>ATFLIWPIYPKIEANEKATAVWLQNTGKTDAMVQIRVFKWNQDGLKDNYSEQSEIIPSPPVAKIKAGEKHMLRLTKSVNLPDGKEQSYRLIVDELPIRLSDGNEQDASKVSFQMRYSIPLFAYGKGIGSGLTEESQKLNAKNALAKPVLQWSVRNNQQGQSELYLKNNGQKFARLSALKTSKTGNDISLGKAAFGYVLSNSTVKFAIDQSTAHELAKTSKIYGVDSSGIKQELIEITKMEDPSGHHHHHH[2x];>[2x]ACSVSASGTSSISVPSIYLMENGENSSQFNSGLSCTGFSLALANMTYLKYRVEQMSNSFTNAQTGEKLNAIILDSNNEIISLGQEKDMSSFTLVNLFSGPDGNLPFYIRLPAGQSVSPGVYQADSPLKVKWFYSVPAVAIVGIGVFFESPGFRRGALGIGFNWGSGADSLGSLSITVLPDCRILAQDVNFGTAAFASKLEPVQSSMGIRCSVNTPYYVSLNNGLSPQNGNQRAMKSQTGNTFLKYDIFKNSSNDRWGSGNERWSSLNATIN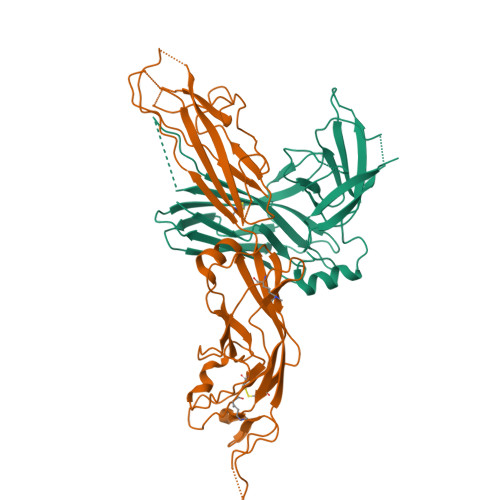PGVHNGVTQQNYVFTTKIVDENADTIPAGTYQDTVTVQVEF>MTALTESSTSKFVKINEKGFSDFNIHYNEAGNGETVIMLHGGGPGAGGWSNYY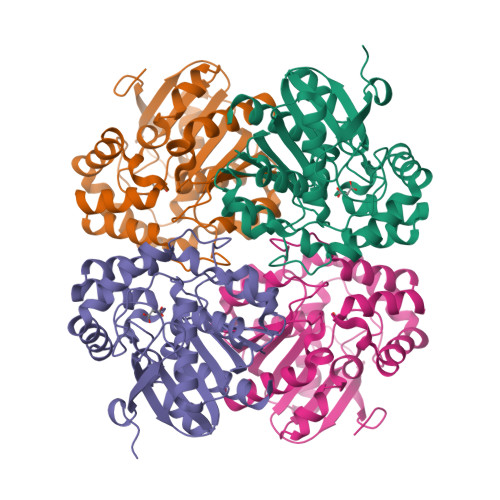RNVGPFVDAGYRVILKDSPGFNKSDAVVMDEQRGLVNARAVKGLMDALDIDRAHLVGNSMGGATALNFALEYPDRIGKLILMGPGGLGPSMFAPMPMEGIKLLFKLYAEPSYETLKQMLQVFLYDQSLITEELLQGRWEAIQRQPEHLKNFLISAQKAPLSTWDVTARLGEIKAKTFITWGRDDRFVPLDHGLKLLWNIDDARLHVFSKCGHWAQWEHADEFNRLVIDFLRHA[2x]> MASIVKTMIVDDSAFMRNILKRILSTTNKYVVIGEAANGADAIKMAEELQPDLISMDI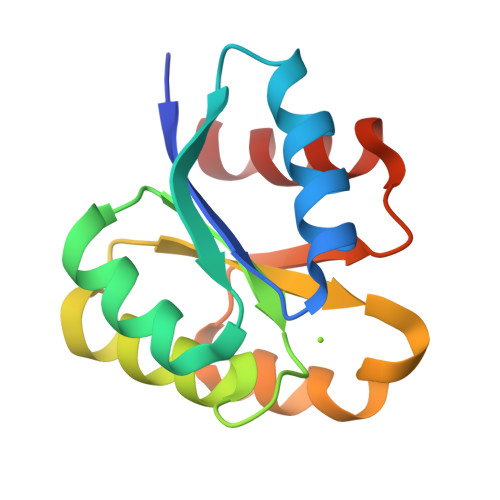VMPETDGITATKAIKEKTPEIKIVMCTSVDQEQKMIDAVNAGADGYIVKPFQAPKILEQFNKLFP>GPLGSAKQQRAEATERVTAGLREVLAARERRAQLEAEGLANLKTLLKVVAVPATVAKTLDQARSAEEIADQVEILVDQTEKARELDVQA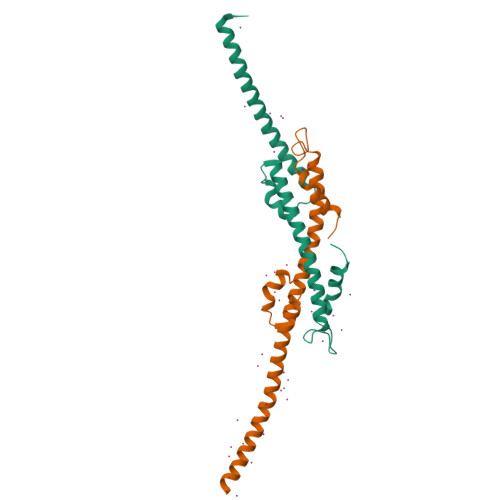VAWLEHAQRTFETHPLSAASGDGPGLLTRQGARLQALFDTRRRVEALRR[2x]NTRs of the importin-α/β class are conserved from yeast to plant cells and transport many distinct cargo proteins into the nucleus. The importin-α armadillo repeat domain binds to nuclear localization sequences (NLSs) of cargo proteins whilst an N-terminal α-helix makes direct contact to importin-β and is therefore called the importin-β-binding (IBB) domain (Cook et al., 2007). The importin-α armadillo repeats form two NLS-binding sites on the concave side of the protein, referred to as ‘major’ and ‘minor’ binding site. Whereas bipartite NLSs make contact to both binding sites, monopartite NLSs bind to either the major or the minor site (Marfori et al., 2011; Chang et al., 2013).

A crystal structure of the MOS6 armadillo repeat domain suggests strong conservation of the NLS-binding sites between MOS6 and four other Arabidopsis importin-αs. We attempted to crystallize ΔIBBMOS6 in complex with either HaRxL106 or an HaRxL106 peptide containing the NLS, but we did not obtain protein crystals of sufficient quality for structure determination. Like other importin-α proteins from yeast, mammals and rice, ΔIBBMOS6 forms 10 armadillo repeats with strong conservation of residues that contribute to the major and minor NLS-binding sites (Marfori et al., 2011). We superposed the ΔIBBMOS6 structure onto the structure of rice importin-α1a in complex with a SV40NLS (Chang et al., 2012). This revealed that essentially all amino acids of rice importin-α1a, that make direct contact to the SV40NLS at the major and minor NLS-binding sites, are conserved in MOS6. We determined the conservation of the NLS-binding sites of importin-αs expressed in rosette leaves by homology modelling based on the ΔIBBMOS6 structure. We found that residues contributing to the MOS6 NLS-binding site are strongly conserved in importin-α1, -α2, -α4 and -α6 whilst these residues are less conserved in importin-α9. However, when only the H3 helices of ARM repeats 1–8 that contribute the NLS-binding sites are considered, the sequence identity is approximately 45% (Wirthmueller et al., 2013). This conservation of the H3 helices allowed us to build homology models for the armadillo repeat domains of other Arabidopsis importin-αs based on the ΔIBBMOS6 structure. Superposition of individual models with the ΔIBBMOS6 structure revealed an almost complete conservation of the major and minor NLS-binding sites in five out of six importin-αs expressed in rosette leaves (importin-α1, -α2, -α3, -α4 and -α6). Our observation that HaRxL106 binds equally well to importin-α1, -α2, -α4 and MOS6 in plant cell extracts is in agreement with a conserved NLS-binding site on these importin-αs.

> MSLRPSAKTEVRRNRYKVAVDAEEGRRRREDNLVEIRKNKREENLQKKRFTSSMAFGSATGQTEQDLSSANQLKDNLPAMVAGIWSEDSNSQLEATNLLRKLLSIEQNPPINEVVQSGVVPRVVKFLSRDDFPKLQFEAAWALTNIASGTSENTNVIIESGAVPIFIQLLSSASEDVREQAVWALGNVAGDSPKCRDLVLSYGAMTPLLSQFNENTKLSMLRNATWTLSNFCRGKPPPAFEQTQPALPVLERLVQSMDEEVLTDACWALSYLSDNSNDKIQAVIEAGVVPRLIQLLGHSSPSVLIPALRTIGNIVTGDDLQTQMVLDQQALPCLLNLLKNNYKKSIKKEACWTISNITAGNADQIQAVIDAGIIQSLVWVLQSAEFEVKKEAAWGISNATSGGTHDQIKFMVSQGCIKPLCDLLTCPDLKVVTVCLEALENILVVGEAEKNLGHTGEDNLYAQMIDEAEGLEKIENLQSHDNNDIYDKAVKILETFWTEDNEEEGNDENHAPQSGFQFGSTNVPPGQFNFI>MGSSHHHHHHSSGLVPRGSHMSATSTATSTSASQLHLNSTPVTHCLSDIVKKEDWSDFKFAPIRESTVSRAMTSRYFKDLDKFAVSDVIIVGAGSSGLSAAYVIAKNRPDLKVCIIESSVAPGGGSWLGGQLFSAMVMRKPAHLFLQELEIPYEDEGDYVVVKHAALFISTVLSKVLQLPNVKLFNATCVEDLVTRPPTEKGEVTVAGVVTNWTLVTQA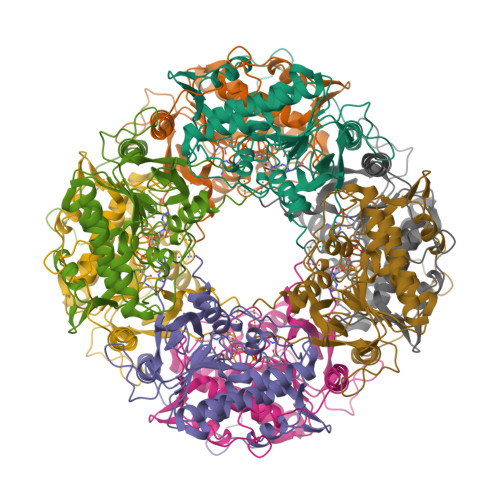HGTQCSMDPNVIELAGYKNDGTRDLSQKHGVILSTTGHDGPFGAFCAKRIVDIDQNQKLGGMKGLDMNHAEHDVVIHSGAYAGVDNMYFAGMEVAELDGLNRMGPTFGAMALSGVHAAEQILKHFAA[4x]N-[2-methyl-3-[4-methyl-6-[4-(4-methylpiperazine-1-carbonyl)anilino]-5-oxo-pyrazin-2-yl]phenyl]-4-(1-piperidyl)benzamide 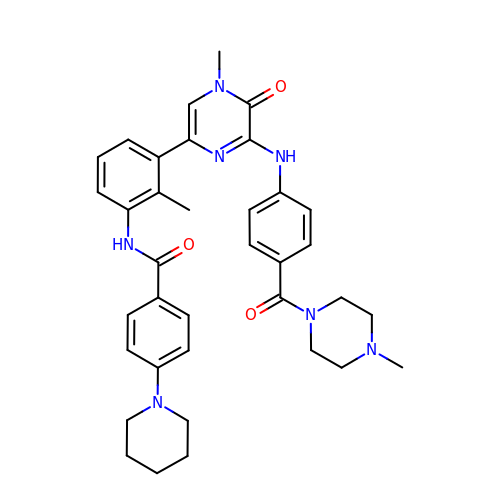| C36 H41 N7 O3 | VDSHGYXLLSEPML-UHFFFAOYSA-N> AELASEKPFRDCADVYQAGFNKSGIYTIYINNMPEPKKVFCNMDVNGGGWTVIQHREDGSLDFQRGWKEYKMGFGNPSGEYWLGNEFIFAITSQRQY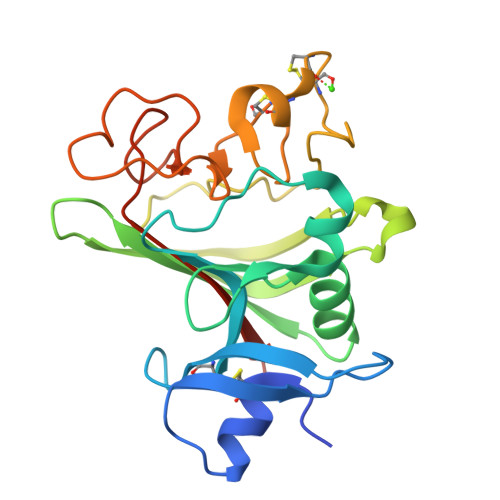MLRIELMDWEGNRAYSQYDRFHIGNEKQNYRLYLKGHTGTAGKQSSLILHGADFSTKDADNDNCMCKCALMLTGGWWFDACGPSNLNGMFYTAGQNHGKLNGIKWHYFKGPSYSLRSTTMMIRPLDFGSLVPR3-Dehydroquinate dehydratase (DHQase) is the third enzyme in the shikimate pathway. DHQase catalyzes the dehydration of 3-dehydroquinate to 3-dehydroshikimate. There are two types of DHQase: type I enzymes catalyze a Schiff base mechanism using a catalytic lysine residue; type II DHQase catalyze the dehydration reaction via an enolate intermediate. DHQase from Enterococcus faecalis is a type I enzyme.

The study also elucidated the structure of E. faecalis DHQase to a resolution of 2.2 Å. The efDHQase monomer has a (β/α)8-barrel scaffold. The majority of the molecule is well ordered and with clear density in the electron density map, with the exceptions of the first and last two residues at the N- and C-terminus, respectively, and a disordered portion (Ala228-Gln236) within the loop connecting the 8th β-strand and the 8th α-helix (β8-α8 loop). There are two monomers in the asymmetric unit of the crystal, forming a homodimer. On each monomer, there are a total of 94 atoms belonging to 24 residues that are involved in the formation of the dimer interface. The non-crystallographic symmetry (NCS) differences for most of the residues are well below 0.3 Å (as reported by COOT), indicating close conformational similarity between the two protomers. Key residues, which are responsible for ligand coordination in the homologous structures, are well conserved in efDHQase (sticks representation). Moreover, these residues, and in particular Lys170, are positioned in nearly identically positions in these three homologous structures, despite the absence of bound ligand in the efDHQase structure. Such similarities strongly suggest that efDHQase catalyzes the dehydration reaction via a Schiff base mechanism whereby the terminal amine of efDHQase's Lys170 reversibly reacts with the carbonyl of the substrate. In the absence of bound ligand, the β8-α8 loop of efDHQase adopts the “open” conformation commonly seen in other DHQases, and becomes partially disordered.

>[2x]GSHMKPVIVKNVRIGEGNPKIVVPIVAPTAEDILAEATASQTLDCDLVEWRLDYYENVADFSDVCNLSQQVMERLGQKPLLLTFRTQKEGGEMAFSEENYFALYHELVKKGALDLLDIELFANPLAADTLIHEAKKAGIKIVLCNHDFQKTPSQEEIVARLRQMQMRQADICKIAVMPQDATDVLTLLSATNEMYTHYASVPIVTMSMGQLGMISRVTGQLFGSALTFGSAQQASAPGQLSVQVLRNYLKTFEQNK> MAELRVLVAVKRVIDYAVKIRVKPDRTGVVTDGVKHSMNPFCEIAVEEAVRLKEKKLVKEVIAVSCGPAQCQETIRTALAMGADRGIHVEVPPAEAERLGPLQVARVLAKLAEKEKVDLVLLGKQAIDDDCNQTGQMTAGFLDWPQGTFASQVTLEGDKLKVEREIDGGLETLRLKLPAVVTADLRLNEPRYATLPNIMKAKKKKIEVIKPGDLGVDLTS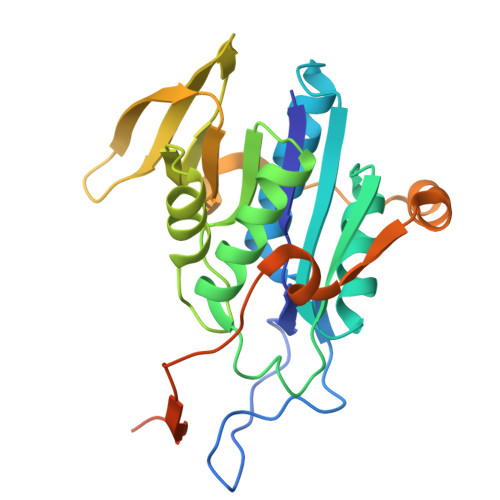KLSVISVEDPPQRTAGVKVETTEDLVAKLKEIGRI> HHHHHHHHENLYF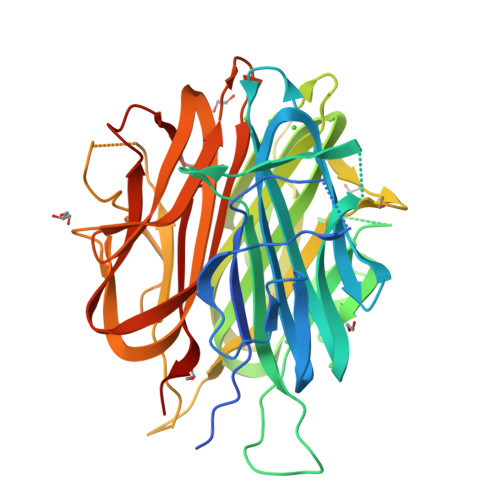QGASPGEGAYVYRSAFSVGLETYVTIPNMPIRFTKIFYNQQNHYDGSTGKFHCNIPGLYYFAYHITVYMKDVKVSLFKKDKAMLFTYDQYQENNVDQASGSVLLHLEVGDQVWLQVYGEGERNGLYADNDNDSTFTGFLLYHDTNPGEGAYVYRSAFSVGLETYVTIPNMPIRFTKIFYNQQNHYDGSTGKFHCNIPGLYYFAYHITVYMKDVKVSLFKKDKAMLFTYDQYQENNVDQASGSVLLHLEVGDQVWLQVYGEGERNGLYADNDNDSTFTGFLLYHDTNPGEGAYVYRSAFSVGLETYVTIPNMPIRFTKIFYNQQNHYDGSTGKFHCNIPGLYYFAYHITVYMKDVKVSLFKKDKAMLFTYDQYQENNVDQASGSVLLHLEVGDQVWLQVYGEGERNGLYADNDNDSTFTGFLLYHDTNGS>MSLTQSSKLIAVIVANIDDYFSTELFKGISSILESRGYIGVLFDANADIEREKTLLRAIGSRGFDGLILQSFSNPQTVQEILHQQMPVVSVDREMDACPWPQVVTDNFEAAKAATTAFRQQGYQHVVVLTSELELSRTRQERYRGILAAAQDVDVLE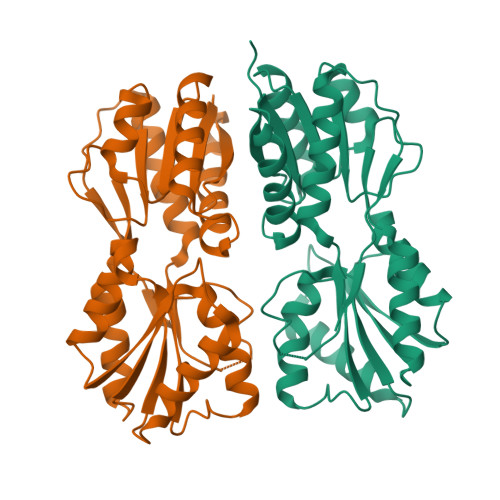VSESSYNHSEVHQRLTQLITQNDQKTVAFALKERWLLEFFPNLIISGLIDNQTVTATGFADTDFIRRMEPKLTLITQNPFLMGASSAEIMLRQLAGEKVAPEKMVIPAKLQEGHHHHHH[4x]3-[4-(methylsulfonylaminomethyl)phenyl]benzoic 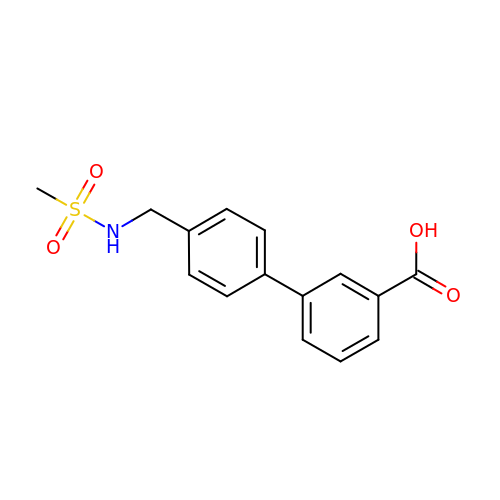acid | C15 H15 N O4 S | GDROHHKTEPPNSN-UHFFFAOYSA-N>[2x]MDSKH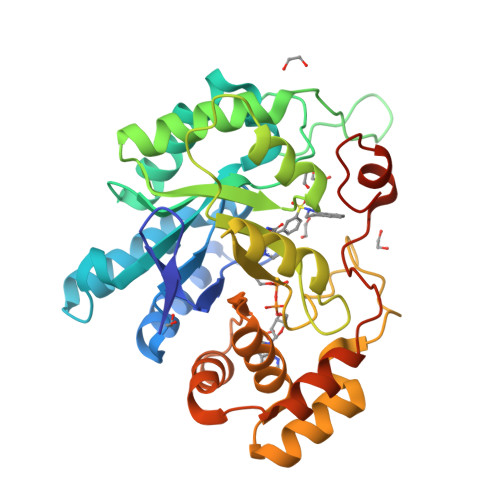QCVKLNDGHFMPVLGFGTYAPPEVPRSKALEVTKLAIEAGFRHIDSAHLYNNEEQVGLAIRSKIADGSVKREDIFYTSKLWSTFHRPELVRPALENSLKKAQLDYVDLYLIHSPMSLKPGEELSPTDENGKVIFDIVDLCTTWEAMEKCKDAGLAKSIGVSNFNRRQLEMILNKPGLKYKPVCNQVECHPYFNRSKLLDFCKSKDIVLVAYSALGSQRDKRWVDPNSPVLLEDPVLCALAKKHKRTPALIALRYQLQRGVVVLAKSYNEQRIRQNVQVFEFQLTAEDMKAIDGLDRNLHYFNSDSFASHPNYPYSDEYLEHHHHHH>[3x]AEIYNKNGNKLDFYGKMVGEHVWTTNGDTSSDDTTYARIGLKGETQINDQLIGYGQWEYNMDASNVEGSQTTKTRLAFAGLKAGEYGSFDYGRNYGAIYDVESATDMLVEWGGDGWNYTDNFMTGRTNGVATYRNSDFFGLVDGLSFALQYQGKNDHDRSIRKQNGDGFSTAATYAFDNGIALSAGYANSNRS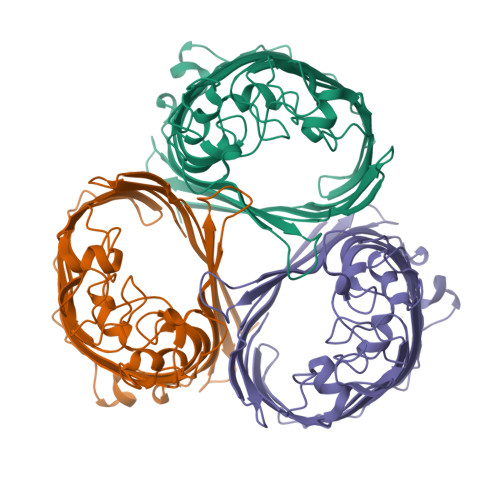VDQKRDGNGDKAEAWATSAKYDANNIYAAVMYSQTYNMTPEEDDHFAGKTQNFEAVVQYQFDFGLRPSLGYVQTKGKNLQARGGFGGGDADLVKYVELGTWYYFNKNMNVYAAYKFNQLDDNAYTRAAGVATDDQAAVGIVYQF Prenyltransferases, also known as isoprenyl diphosphate synthases, catalyze the sequential condensation of a basic five-carbon building block (C5), the isopentenyl diphosphate (IPP), to synthesize prenyl precursors of isoprenoid metabolites and isoprene polymers, collectively called polyisoprene. Ultrahigh molecular weight cis-1,4-polyisoprene and trans-1,4-polyisoprene (TPI), which are the principal components of natural rubber and gutta-percha, respectively, are also isoprenoid metabolites that are assumed to be synthesized by specialized prenyltransferases. These prenyltransferases are divided into two major groups, the cis-1,4-prenyltransferases (CPTs) and trans-1,4-prenyltransferases (TPTs), based on the stereochemistry of the double bond formed during IPP condensation. To investigate the molecular properties of the EuTPT proteins, we determined the three-dimensional structures of EuTPT3 and EuFPS1 using X-ray crystallography. Similar to EuFPS1 and other prenyltransferases, the EuTPT3 subunits were composed of 10 core helices (α1-α10) with a deep pocket that included two DDxxD motifs responsible for substrates binding.

Specifically, the equivalent positions of residues Cys94 and Ala95 on α4 in EuTPT3 are occupied by Tyr88 and Phe89 in EuFPS1. Therefore, those residues were predicted to be critical for the α5 arrangement and dimeric architecture. To test this hypothesis, we replaced Cys94 and Ala95 in EuTPT3 with tyrosine and phenylalanine, respectively, to create the double mutant EuTPT3(C94Y/A95F). An in vitro test demonstrated that the double mutant lacked the activity for synthesizing ultrahigh molecular weight TPI. Interestingly, we determined the crystal structure of the EuTPT3(C94Y/A95F) mutant protein at 3.3 Å resolution and found that it formed the FPS dimeric conformation. The mutated residues changed the orientation of α5, compared with that in the wild type. The RMSD values of the double mutant subunit compared to the wild-type structures of EuTPT3 and EuFPS1 were 3.41 Å (no. of Cα = 202) and 1.85 Å (no. of Cα = 284), respectively. Thus, the replacement of only two residues switched the dimeric conformation from the TPT-type to the FPS-type dimer. Actually, the replacements of the exact two amino acids in other EuTPTs and their endo product analysis provided reasonable results; mutations of Cys94 and Ala95 in EuFPS1 and Cys96 and Ala96 in EuTPT5 to Tyr and Phe, respectively, resulted in synthesizing FPP, whereas Tyr88 and Phe89 in EuTPT2 (EuFPS1) and Phe95 and Phe96 in EuTPT4 (EuFPS2) produced longer chain length end-product than FPP. These results indicated that Cys94 and Ala95 on α4 in EuTPT3 and the corresponding amino acid in other EuTPTs were essential for the TPT-dimer conformation, which forms the path for newly synthesized ultrahigh molecular weight TPI. Thus, those two residues not only play a key role in determining the product length but also in the formation of the TPT-type dimer.

>MNHKVHHHHHHIEGRHMTELKSKFVKVYSVLKKELLHDSAFGLTDDSRNWVERIMDYNVPGGKLNRGLSVVDSYKLLRELTGGKSELSDDEIFLASVLGWSVEWIQAYFLVLDDIMDHSHTRRGHPCWFRLPKVGMIAINDGLILRNHVPRILRTHFQTEHYYLQLVDLFHEVECQTIAGQMLDLITTLAGEINLSSYSLPVYQQITLSKTSYYSFYLPVACALVMLGENLESHDDMKDILLEMGTYFQVQDDYLDCFGDPEVIGKIGTDIEDNKCTWLVVQALEHCNEEQKKLLYDNYGRKDPKQVAKVKELYKTLNLEDLFTQYENKTCKKLTKSIEALPNVAVQAVLKSFLAKIHKRLK[2x]> MHHHHHHENLYFQGSSIYPPETSWEVNKGMNSSRLHKLYSLFFDKSSAFYLGDDVSVLEDKPLTGAYGFQSKKNDQQIFLFRPDSDYVAGYHVDAKSDAGWVNDKLDRRLSEISEFCSKATQPATFILPFVEMPTDITKGVQHQVLLTISYDPKSKQLTPTVYDSIGRDTYSESLSSYFKGKYRTTCDEILTQSIEKAIKSTDFTLGKFTRAAYNHQNRLTEGNSGSYTFRTIKEVISSSAQGTEVKIPGSGYITSNSYLTS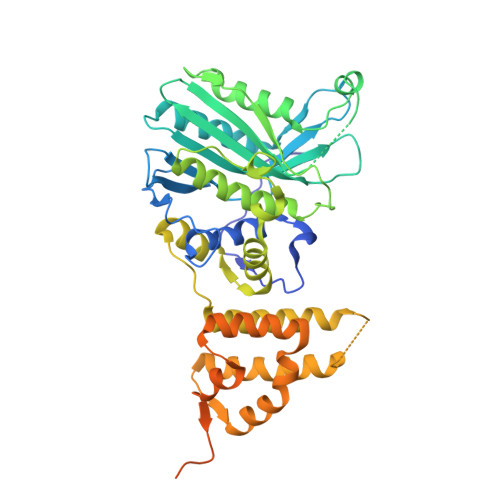QHVQDIESCIKYRNLGVVDIESALTEGKTLPVQLSEFIVALEDYGKLRSQQSEKSMLNFIGYSKTAKLTAVELLIGILNDIKGKNEISESQYDKLVKEVDCLMDSSLGKLVQFHLKNLGAESLQKLVLPCVKFDDTIDDFVTIEKDELFDVPDITGEELASKKGIEQGALDKEALLKQKQIKTDLLDLREEDKTGLKKPLHGGIKVK>MAEKPKLHYSNIRGRMESIRWLLAAAGVEFEEKFIKSAEDLDKLRNDGYLMFQQVPMVEIDGMKLVQTRAILNYIASKYNLYGKDIKEKALIDMYIEGIADLGEMIGDLSFSQPEEQDAKLALIQEKTKNRYFPAFEKVLKSHGQDYLVGNKLSRADIHLVELLYYVEELDSSLISSFPLLKALKTRISNLPTVKKFLQPGSPR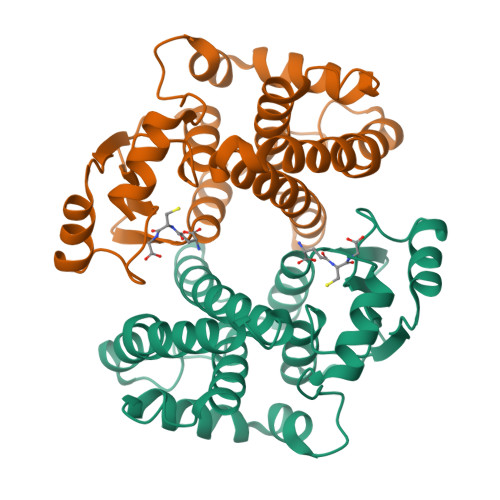KPPMDEKSLEESRKIFRH[4x]> MKVEEILEKALELVIPDEEEVRKGREAEEELRRRLDELGVEYVFVGSYARNTWLKGSLEIDVFLLFPEEFSKEELRERGLEIGKAVLDSYEIRYAEHPYVHGVVKGVEVDVVPCYKLKEPKNIKSAVDRTPFHHKWLEGRIKGKENEVRLLKGFLKANGIYGAEYKVRGFSGYLCELLIVFYGSFLETVKNARRWTRRTVIDVAKGEVRKGEEFFVVDPVDEKRNVAANLSLDNLARFVHLCREFMEAPSLGFFKPKHPLEIEPERLRKIVEE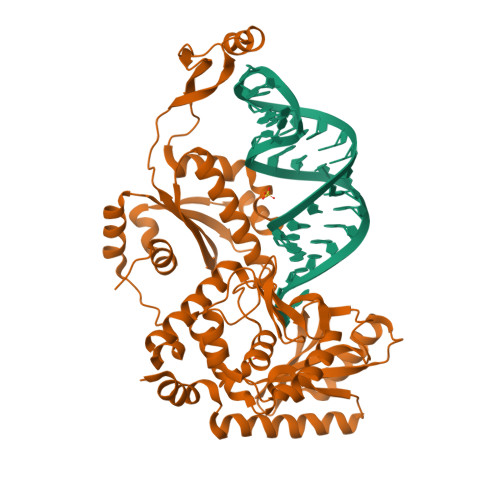RGTAVFAVKFRKPDIVDDNLYPQLERASRKIFEFLERENFMPLRSAFKASEEFCYLLFECQIKEISRVFRRMGPQFEDERNVKKFLSRNRAFRPFIENGRWWAFEMRKFTTPEEGVRSYASTHWHTLGKNVGESIREYFEIISGEKLFKEPVTAELCEMMGVKD> MAPAPPANSGESSLLSESELPAGISYAEAMEGGSRPLLHPDNPVVFFDISIGSHEAGRIKIELFKNLAPKSAENFRQFCTGEFRQNQVPIGYKGATFHRIIKNFMIQGGDFVKGDGTGRLSIYGSSFPDEAFVLPHFRSGLLSLANSGPDTNGCQFFITCAKCDWLNRKHVVFGQVLGKESMQVVRKIEHVTVDGGNRP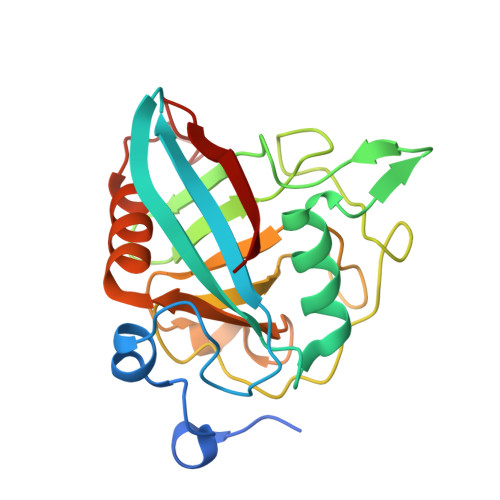RIPVTVTQCGEL7-fluoranyl-~{N},~{N}-dimethyl-1-benzofuran-2-carboxamide | C11 H10 F N 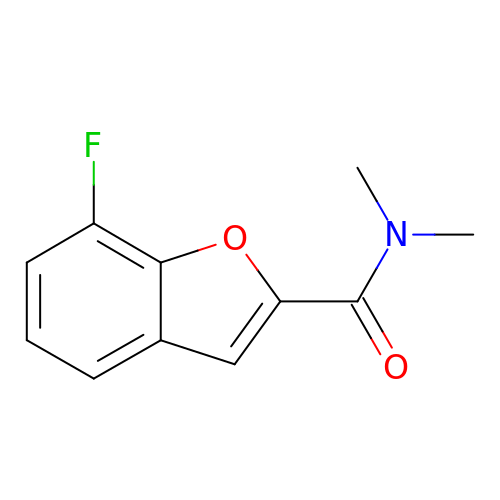O2 | ASMPIWMZHMGTON-UHFFFAOYSA-N> MGDTTQLVKEYQEKRSKLEKF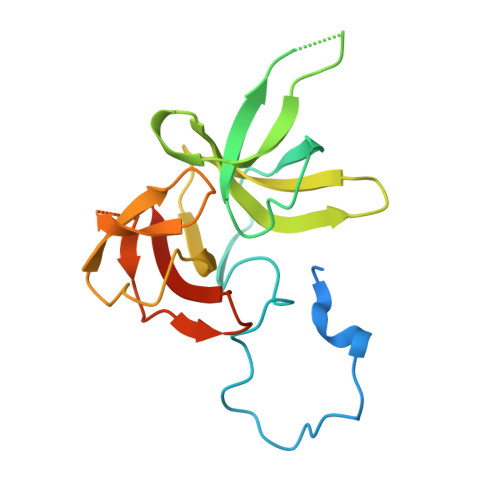MKNPQHDASLLSNSNEFRDKNVEFFASGGTRTSKFDKLENHPFLGYPYKRGVKRVIQEAQDNQSHYEPHVEAGGGEDLYGICIDIDEFSKTATIVPITNNFEGYLVAKDSTVKVKDKLIFNKDGALEKVTGAPNKATINATALTDAKQISNEVYLVKVAVFGNKAMSRN> GKKAVINDSNTPLHLL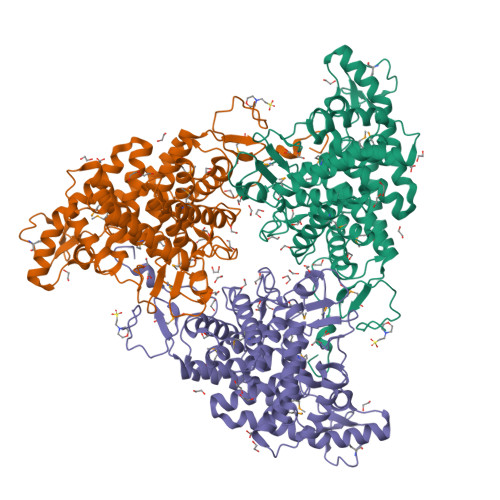QPAYQGTYGDLTPEQVKKDIDRVFAYIDKETPARVVDKNTGKVITDYTAMGDEAQLERGAFRLASYEWGVTYSALIAAAETTGDKRYTDYVQNRFRFLAEVAPHFKRVYEEKGKTDSQLLQILTPHALDDAGAVCTAMIKLRLKDESLPVDGLIQNYFDFIINKEYRLADGTFARNRPQRNTLWLDDMFMGIPAVAQMSRYDKEAKNKYLAEAVKQFLQFADRMFIPEKGLYRHGWVESSTDHPAFCWARANGWALLTACELLDVLPEDYPQRPKVMDYFRAHVRGVTALQSGEGFWHQLLDCNDSYLETSATAIYVYCLAHAINKGWIDAIAYGPVAQLGWHAVAGKINEEGQVEGTCVGTGMAFDPAFYYYRPVNVYAAHGYGPVLWAGAEMIRLLNTQHPQMNDSAVQYYQEKQKTTAPIFAVDSE>[2x]ATPVKVY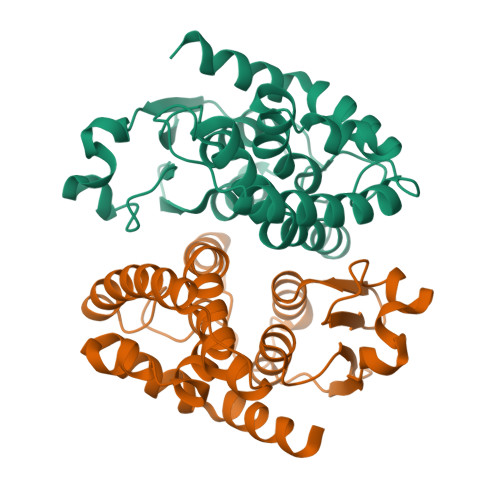GPPLSTAVSRVLVTLLEKDVPFQIIPVDMSKGEHKKPDYLKIQPFGQVPAFQDESISLFESRSICRYVCEKYADRGDKGLYGTNPLERASIDQWVEAEGQSFGPSSGALVFQLAFAPRMNIPQDQGVIKQNEEKLGKVLDIYEQRLGESRFLAGDEFTFADLSHLPNGDYLVNATDKGHLFTSRENVGRWWNEISDRESWKKVIEMRKSG> 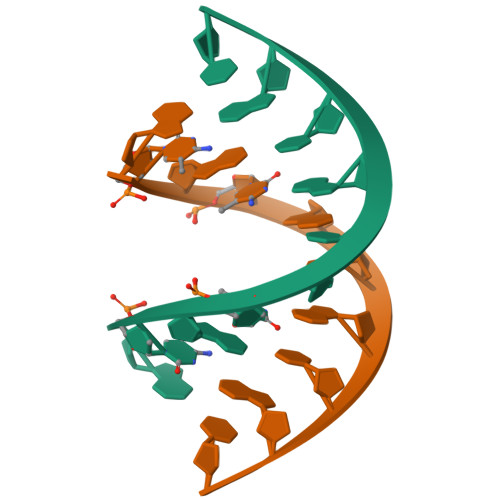GCGCGCGCGC4-[[(4R)-5-cyclopentyl-4-ethyl-3a,4-dihydro-3H-[1,2,4]triazolo[4,3-f]pteridin-7-yl]amino]-N-cyclopropyl-3-methoxy-benzamide 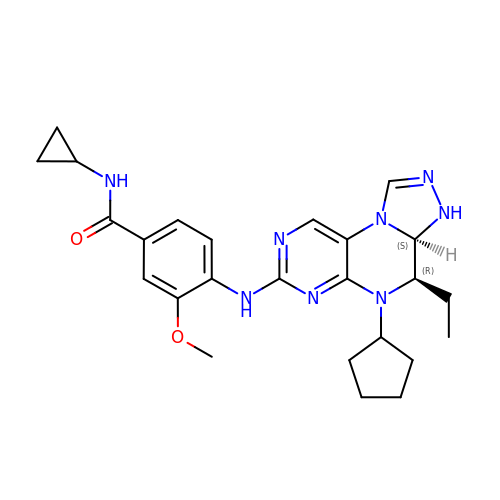| C25 H32 N8 O2 | BNAAGNVFCJFJIF-AUSIDOKSSA-N> GSHMKTMIYPHQYNYIRSVILRLKNVYKTVNDKETVKVIQSETYNDINEIFGHIDDDIEESLKVLMNIRLSNKEIE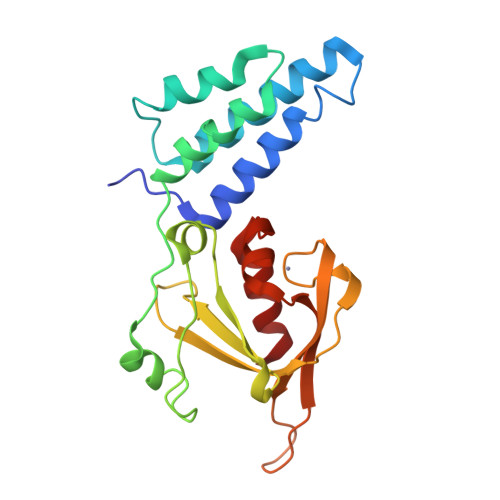AILNKFLEYVVPFELPSPQKLQKVFKKVKKIKIPQFEEYDLKVSSFVGWNELASNRKYIIYYDEKKQLKGLYGEISNQVVKGFCTICNKESNVSLFMKKSKTNSDGQYVKKGDYICRDSIHCNKQLTDINQFYNFIDKLD> MGNDDIRQVYYRDKGISHAKAGRYSQAVMLLEQVYDADAFDVDVALHLGIAYVKTGAVDRGTELL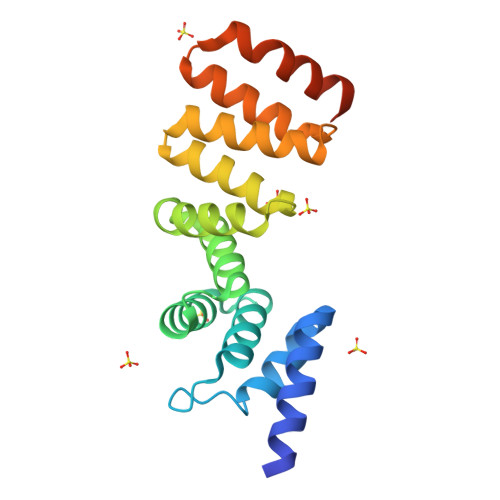ERSLADAPDNVKVATVLGLTYVQVQKYDLAVPLLIKVAEANPINFNVRFRLGVALDNLGRFDEAIDSFKIALGLRPNEGKVHRAIAFSYEQMGRHEEALPHFKKANELDEGASVELALVPR>[2x]GLNGGSQTCNFNNAL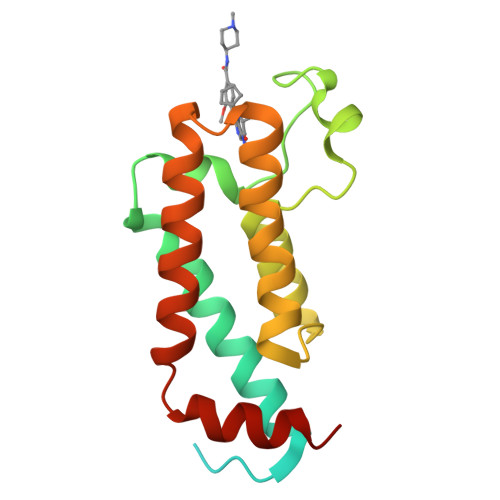NPSNGGAGLHISNNLDGSHNVINAGPNITSYTEALDEFCIELQRIINSTKTLHHYSHVFWNRVSERIAPNYYNLVKRPMWLQLMINKCKKREYKSRKDFQDDLDLIVENCKIYNGVNHPLVSVATLIHSNVVKKIDEIQGIEKIEAYLSLKP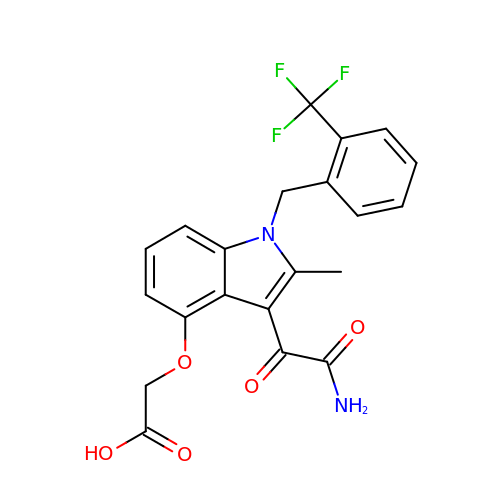2-[2-methyl-3-oxamoyl-1-[[2-(trifluoromethyl)phenyl]methyl]indol-4-yl]oxyethanoic acid | C21 H17 F3 N2 O5 | AKFUWCKNXCSWDQ-UHFFFAOYSA-N> AMALTGCSEKININEDKISHKIDIPDSAWTIGIGEKFKNAGHPNVKYPMIDDSYVQGAPLGGFGAGTIGRTYNGGFSRWHLEIGKNKYTTVYANQFSVFQKVEGNKDGVAQVLYAGEPENGYLSSWKWDYPKESGMYYALYPNSWYTYTNKDLPVQLAVKQFSPIIPYNYKETSYPVAVFKWTAYNPTNKNVDVSIMFTWQNMIGFFGKQVNVNSGNFNKIIKDKSKDSEIVAAVMGNISNDNEEWNGEYSIGVKKVPGVDISYKAKFVTTGDGSDLWHEFSKNGILDNKDDETPTKQDGIGSAIAVNFKLQPGQTIEVPFALSWDLPIMKFGGGDKWYKMYTKYFGKNGKNSFAILKEALNNYQKWEKMIDDWQKPILSNKSKPDWYKTALFNELYYLADGGTAWENGKVGEKDKRTNNMFGLLACFDYNYYETLDVRFYGSFPLVMLWPDIEKQVMRQFADTINVQDSSEFKVGSNGAMAVKKVQGMIPHDLGSSYALPWIKINAYDWQNPNIWKDLNSKYVLLVYRDYVLTGKTDKEFLKYTWKSVKTALDKLKEMDKDNDGIPDNEGIPDQTYDTWSMKGTSAYC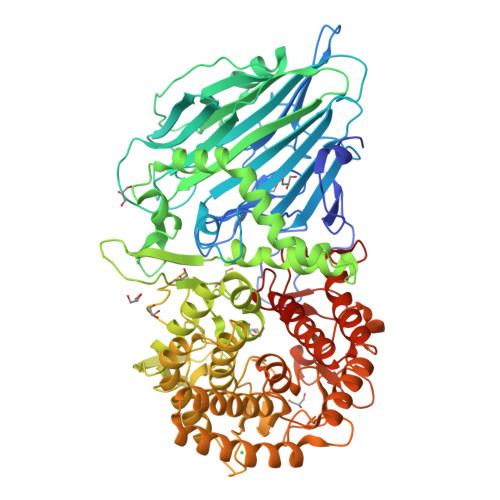GSLWLAALKAAQEIGKVLKDNEAYIKYNEWYKIAQQNFEKELWNGEYYNFDTESDHKDSIMADQLAGQWYADILRLGDILPKDHVQKALKKIYEFNVMKFENGKMGAVNGMRPDGIVDESDIQAQEVWTGVTYALASFMKYRGMTEEAYNTAYGVYKMTYDKSGKGYWFRTPEAWTKDGNYRASMYMRPLSIWSMEVNYNEVLEHHHHHH Later, Hop2 and Mnd1 were found to work together as a complex that promotes homologous chromosome pairing and DSB repair during meiosis. It greatly promotes the Dmc1- and Rad51-mediated strand exchange between the presynaptic filament and recombining double-stranded DNA (dsDNA) to form a D-loop, suggesting that this activity of Hop2–Mnd1 may be responsible for the synaptic complex formation only between homologs during meiosis. In order to provide structural information of the entire Hop2–Mnd1 complex at atomic resolution and to understand the mechanistic aspects of the Hop2–Mnd1 function, we have determined the crystal structure of full-length Hop2–Mnd1 derived from Giardia lamblia. The structure reveals that the WHDs of Hop2 and Mnd1 are closely juxtaposed via evolutionarily conserved interdomain interactions—thereby forming a joint dsDNA-interacting interface—and attached to an elongated, crescent-shaped Dmc1-binding structure.

The heterodimeric complex of full-length G. lamblia Hop2 (231 residues) and Mnd1 (203 residues) was crystallized subsequently. After extensive crystal screening to collect suitable X-ray data sets, the structure of Hop2–Mnd1 was determined by the single wavelength anomalous dispersion method using a selenomethionine-derivatized crystal. The asymmetric unit of the crystal contained three copies of Hop2–Mnd1. Only one Hop2–Mnd1 heterodimer, referred to as Heterodimer I, exhibited electron densities for nearly the entire length of the molecules. The N-terminal ∼70 residues of both Hop2 and Mnd1 fold into winged-helix domains (WHDs) that are juxtaposed to each other through conserved interactions. The following 161 residues of Hop2 and 131 residues of Mnd1 both fold into three α-helices that are interrupted by two short non-helical regions. These α-helices of the two proteins together form a parallel coiled coil that provides the major interface for heterodimer formation. Finally, the C-terminal segments of Hop2 and Mnd1 fold back onto the C-terminal leucine zipper (LZ3) to form a helical bundle-like structure, which is designated as LZ3wCH (for LZ3 with capping helices). With these dimensions, the overall structure of Hop2–Mnd1 is an elongated rod, which is curved due to the two kinked junctions. Presumably, the overall curved rod-like structure observed in the crystal is likely to be the inherent molecular shape of Hop2–Mnd1 under physiological conditions, while it is conformationally flexible at the three junctions to some degree.

>MAPKGTSLDEKKERLLEEMLKRGEIYSNKTIETLSKPTGISSMVIKNVLQALVNEDLVDTDKIGASTYYWCFASKRSQAARTELARLQKALEEQTNFIDKATARIEELKVGREETEERSSLLKEKLALQVKLEEQRGTFRDLLKNDPDVAQKLRNYTDIAKQEANLWTDNIFCLQKYMLTKLQMDKKTVSTALGITGEFDYLE[3x];>[3x]MAAAYKEAFAAVKELMQTSNKPQNVQTAINNTGSKYGKTTVQKALDELVAQNLCIYTEIGKTGKLYLWNQNLLEVLSDAQLMEVNAQINDLKAQVEKLTQQGETLRITQRNLEAAPITEVLKQEVDELRQQVSANDEKLRLVRESNAIVSDADMLTLQKNYKDAMTAWATRRAKCREVIDTLSEGMGVKPSAFMDQLGLEEGLPMTTYTEMKKALPPVNVSKADIKAALKK>GPSSPSLLRAIPGIAWIALLLLVIFYVFAVMGTKLFAQSFPEWFGTLGASMYTLFQVMTLESWSMGIARPVIEAYPWAWIYFVSFILVSSFTVLNLFIGIIIESMQSAHWEGGGAKRIEQEQRAHDERLEMLQLIRDLSSKVD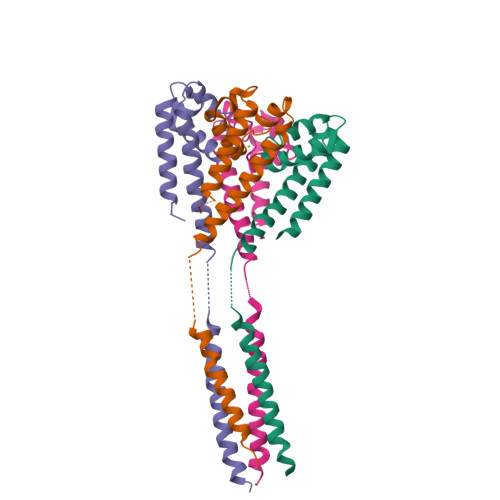RLERRSGKR[4x]> 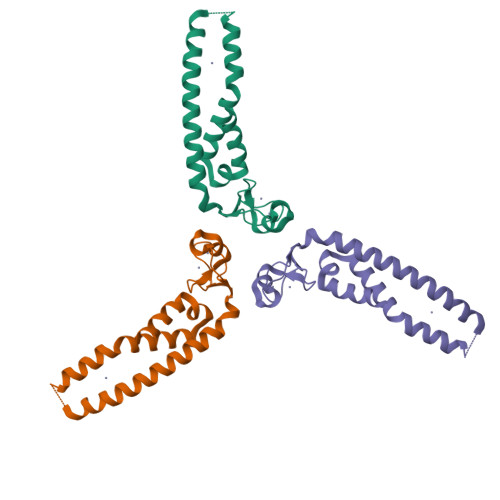EEGQKVDHCAHHGEKLVLFCQQDGNVICWLCERSQEHRGHQTFLVEEVAQKYREKLQVALEMMRQKQKDAETECNQVAKRVPKAPPEEKEALIARGKACGEQTQSVRVLISDLEHRLQGSVMELLQGVDGVIKRIEKVTLQ N-(2-{[(4-chlorophenyl)methyl]disulfanyl}ethyl)decan-1-amine 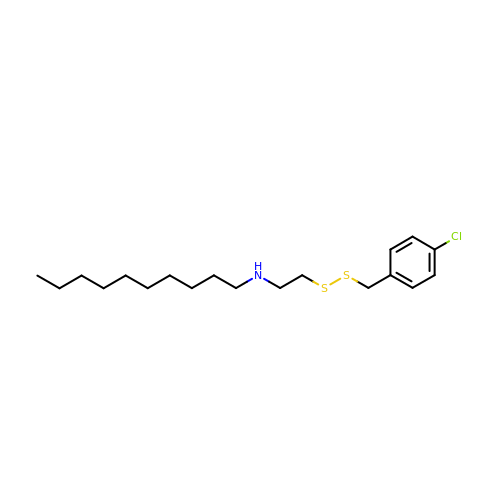| C19 H32 Cl N S2 | MTCITSZEZJBERN-UHFFFAOYSA-N8-DEMETHYL-8-DIMETHYLAMINO-FLAVIN-ADENINE-DINUCLEOTIDE | C28 H36 N10 O15 P2 | 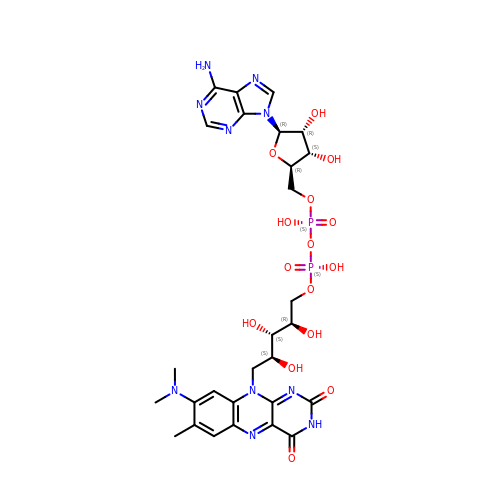UXOZEHHQWXVTPI-MZWSMYJRSA-N>[4x]MKVRVKAPCTSANLGVGFDVFGLCLKEPYDVIEVEAIDDKEIIIEVDDKNIPTDPDKNVAGIVAKKMIDDFNIGKGVKITIKKGVKAGSGLGSSAASSAGTAYAINELFKLNLDKLKLVDYASYGELASSGAKHADNVAPAIFGGFTMVTNYEPLEVLHIPIDFKLDILIAIPNISINTKEAREILPKAVGLKDLVNNVGKACGMVYALY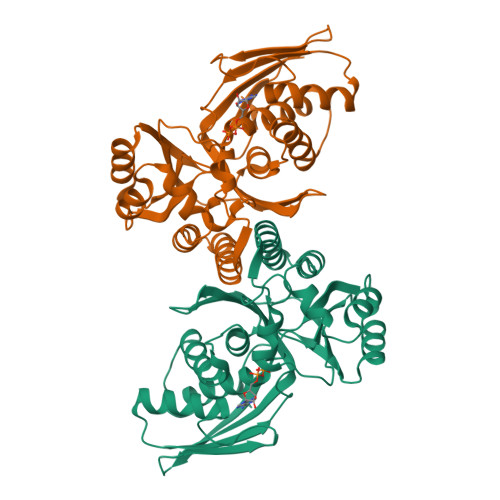NKDKSLFGRYMMSDKVIEPVRGKLIPNYFKIKEEVKDKVYGITISGSGPSIIAFPKEEFIDEVENILRDYYENTIRTEVGKGVEVV>GIDPFTAVAAPSPAAAAEPGPAARPRSTRGQVRLPGGEFAMGDAFGEGYPADGETPVHTVRLRPFHIDETAVTNARFAAFVKATGHVTDAERFGSSAVFHLVVAAPDADVLGSAAGAPWWINVRGAHWRRPEGARSDITGRPNHPVVHVSWNDATAYARWAGKRLPTEAEWEYAARGGLAGRRYAWGDELTPGGRWRCNIWQGRFPHVNTAEDGHLSTAPVKSYRPNGHGLWNTAGNVWEWCSDWFSPTYYAESPTVDPHGPGTGAARVLRGG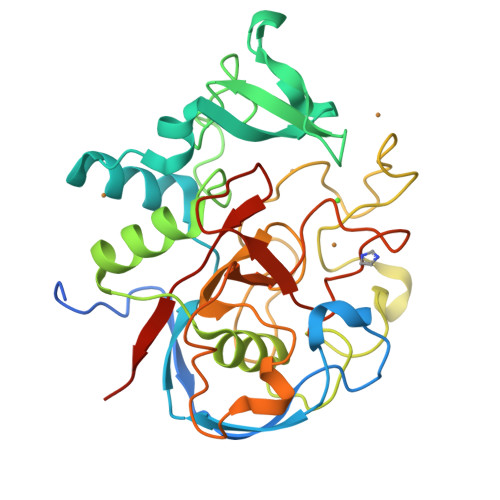SYLCHDSYCNRYRVAARSSNTPDSSSGNLGFRCANDADLTSGSAAE[5x]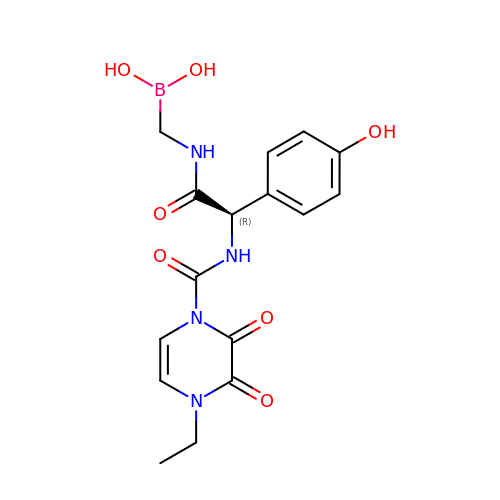({[(2R)-2-{[(4-ethyl-2,3-dioxo-3,4-dihydropyrazin-1(2H)-yl)carbonyl]amino}-2-(4-hydroxyphenyl)acetyl]amino}methyl)boronic acid | C16 H19 B N4 O7 | VFZCHJQIIUDDPB-GFCCVEGCSA-N> GSSGSSGLDAVSQAAQKYEALYMGTLPVTKAMGMDVLNEAIGTLTARGDRNAWVPTMLSVSDSLMTAHPIQAEASTEEEPLWQCPVRLVTFIGVGRDPHTFGLIADLGRQSFQCAAFWCQPHAGGLSEAVQAACMVQY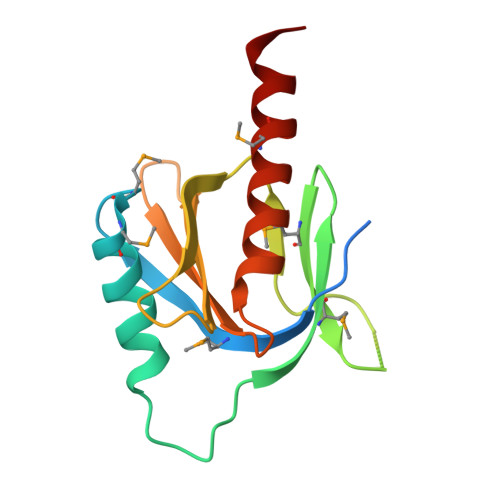QKCLVA>CGCGCG[4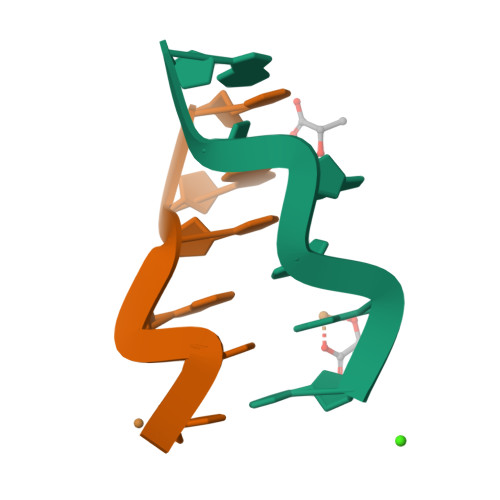x]>MYMKFTYHFHAYQPGDIIYVHDGSGWDPIKYSERLSPVALEIREEEVKGRNWTRAMIKAYEYVDETLRMLDEGAVSVDFEPFTLYMVLKYKPKIYGEIVETLETHVEPTVTVPFHPIMPHLSHFEQEILSKVSFDFYLPFIARKPIVSFWLPENVITKDTAKIVTSATDKDVVFLLDERQFIGVNIPQARFSCNKYLCDGKSAFVFGRIHYISDAFAFNTLDVEGLTRAVAEGCVDVFKEKEGIEYLVFLSSDLESLVANPKQLDRFLGWIDGLKKRGIEIINVAEFIRKKVSNEYKSLPGECSESFRINVKDYSSWSDYFDLSVDGRTSDMRWTGIRREDNVVIHRWYKERKVSQLWKFAFMKLFRELNRAVRFGVIDMLRTQGVSDIEKIKEFLVRYSRVFFREHYEYFELDTSVDYVMEPIHEADPSLALKLGRIYYLMLLANHSCPRFWENI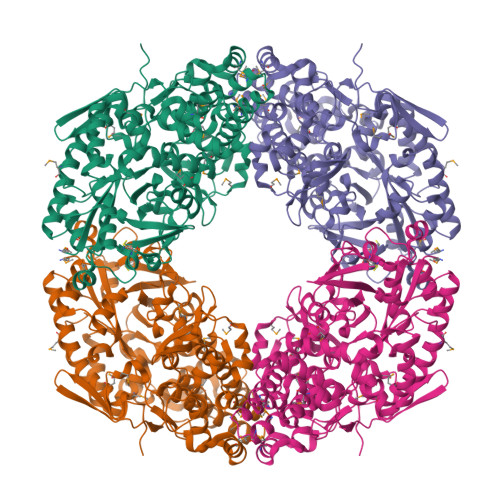DTRVTFGNVATISKALIELMELYMEENEERANYIFLEYMKLLAFPQLYYDYDLFRMKGLEGWETTEKAWFESLRSEVPNSKYNVVTRAALYVGKRDLPPDMRSVIDTLYDLEEAVPDTGHIPGEMHGKWENKEWCEHKGKD[2x]(4R,5S)-3-((2R,3S,4S)-2-ethyl-5-((2R,3R)-2-ethyl-3-(2-((2R,3R)-2-ethyl-3-methyloxiran-2-yl)ethyl)oxiran-2-yl)-3-hydroxy-4-methylpentanoyl)-4-methyl-5-phenyloxazolidin-2-one 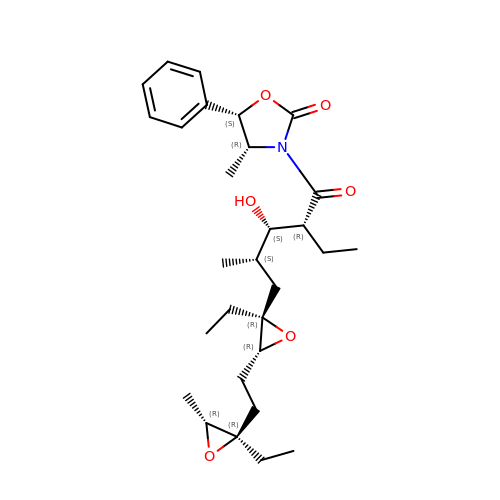| C29 H43 N O6 | PLMSSXURLNIBST-CWZDORBJSA-N Bacterial HSS is mostly found in α-proteobacteria and in some β- and γ-proteobacteria, including pathogenic strains such as Legionella pneumophila, Brucella spp. and various P. aeruginosa strains, including PA7 and PA14. It catalyzes the conversion of two molecules of putrescine (PUT; 1,4-diaminobutane) into one molecule of sym-homospermidine [HSP; bis(4-aminobutyl)amine] as the main reaction along with several side reactions (Ober et al., 1996; Böttcher et al., 1994). Bacterial HSS is NAD+-dependent, active at neutral to basic pH with an optimum at pH ∼8.8, and shows increased activity in the presence of 50 mM potassium ion. BvHSS forms a dimer, with each subunit containing a boot-shaped substrate-binding pocket between an NAD(P)-binding Rossmann-like domain and an HSS-like domain. The cofactor NAD+ is bound as a prosthetic group in the binding pocket with its nicotinamide ring being part of the active site.

Krossa and coworkers identified three binding sites for the amino groups of reaction components within the substrate-binding pocket. Assuming the amino groups of the reaction components to be protonated at neutral to slightly basic pH, the ‘innermost’ N atoms of PUT (N1) and of HSP (N01) mainly bind via a salt bridge to Glu210 and, in addition, via a hydrogen bond to Asn162 at the ‘inner amino site’. Following a similar approach to probe the role of BvHSS residue Glu210, the E210A, E210Q and E210K variants were examined and were found to be inactive. Superimposition of the variant structures onto the wild-type structure revealed nearly identical locations of all residues in the binding pocket, including the wild-type and variant residues Glu210 and Gln210. These findings convincingly demonstrate the indispensable need for a negative charge at position 210 to stabilize the positively charged amino groups of the reaction component at the ‘inner amino site’.

>[2x]GPMGTDWPVYHRIDGPIVMIGFGSIGRGTLPLIERHFAFDRSKLVVIDPSDEARKLAEARGVRFIQQAVTRDNYRELLVPLLTAGPGQGFCVNLSVDTSSLDIMELARENGALYIDTVVEPWLGFYFDPDLKPEARSNYALRETVLAARRNKPGGTTAVSCCGANPGMVSWFVKQALVNLAADLGVTGEEPTTREEWARLAMDLGVKGIHIAQRDTQRASFPKPFDVFVNTWSVEGFVSEGLQPAELGWGTFERWMPDNARGHDSGCGAGIYLLQPGANTRVRSWTPTAMAQYGFLVTHNESISIADFLTVRDAAGQAVYRPTCHYAYHPCNDAVLSLHEMFGSGKRQSDWRILDETEIVDGIDELGVLLYGHGKNAYWYGSQLSIEETRRIAPDQNATGLQVSSAVLAGMVWALENPNAGIVEADDLDFRRCLEVQTPYLGPVVGVYTDWTPLAGRPGLFPEDIDTSDPWQFRNVLVRD>SNAMFQTTSNFGIVVEQHLRRISFFSTDTLEILNQITLGYDFVDTAITSDCSNVVVTSDFCQTLVQIETQLEPPKVVAIQEGQSSMADVDITPDDQFAVTVTGLNHPFNMQSYSFLKNKFISTIPIPYDAVGIAISPNGNG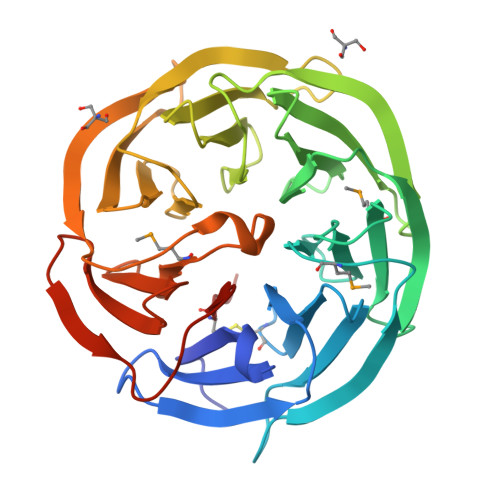LILIDRSSANTVRRFKIDADGVLFDTGQEFISGGTRPFNITFTPDGNFAFVANLIGNSIGILETQNPENITLLNAVGTNNLPGTIVVSRDGSTVYVLTESTVDVFNFNQLSGTLSFVKSFGHGLLIDPRPLFGANQMALNKTETKLFISANISRELKVFTISGKVVGYVAGIEANGGIAICHPDKHNRLK[2x]>MSFVPFLEPFIPHENTL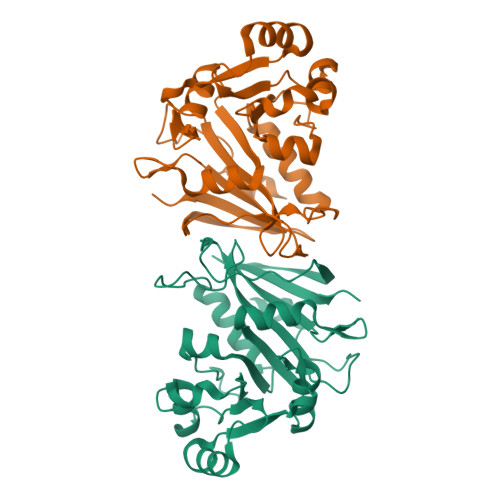LPELPFVTLTYAQSLDSRIAAKKGERTVISHQETKNMTQYLRSKHDAILVGVKTVLADDPGLNCKLGTPIRPIILDPTFQLLSKIASLKLIKLGLSGEGEPPVFITRKGVVSPDLQANLRSDYGISIVEIADRDVHRGKMSWFAILKILKDAEIHSVMVEGGATIINDLLICRQNSVPLVASLIITVGPVYLGKDGVEVTPARSVKLGNVRWWHGIQDAVVAASLELEHHHHHH[2x]>PAFVNKLWSMVNDKSNEKFIHWSTSGESIVVPNRERFVQEVLKKYFKHSNFASFVRQLNMYGWHKVQDVKSGSMLSNNDS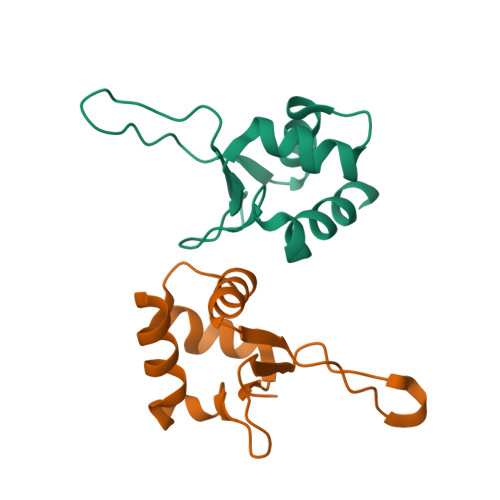RWEFENERHA[2x]Mupirocin, a clinically used natural antibiotic, inhibits isoleucyl-tRNA synthetase (IleRS), an enzyme that links isoleucine to its tRNAIle for protein synthesis. Two IleRSs, mupirocin-sensitive IleRS1 and resistant IleRS2, coexist in bacteria. Specifically, type 1 proteins (IleRS1) are strongly inhibited by mupirocin (Ki in low nanomolar range), while IleRS2, which are homologous to IleRSs from the eukaryote cytosol, exhibit resistance to mupirocin concentrations that are about three orders of magnitude higher. AARSs catalyze the formation of AA-tRNA in two steps within the same active site. The amino acid is first activated by ATP to form an aminoacyl-adenylate (AA-AMP) intermediate, followed by the transfer of the aminoacyl moiety to the tRNA.

To understand how IleRS2, but not IleRS1, accommodates the non-canonical motif, we used X-ray crystallography to determine the structures of a pair of IleRS enzymes from the same organism. Apart from wild-type PmIleRS1 and PmIleRS2, both of which harbor the canonical HXGH motif, we also structurally characterized their corresponding GXHH mutants, all in complex with a non-hydrolyzable analog of the isoleucyl-adenylate reaction intermediate, Ile-AMS. Additionally, the structure of the C-terminal tRNA anticodon binding domain, which differs among the two IleRS types, is resolved for a type 2 protein. However, superimposing the HUP catalytic cores of IleRS1 (residues 50–174 and 523–635) and IleRS2 (residues 40–168 and 513–632) unraveled conformational rearrangements within the signature motifs in the active sites. Relative to IleRS1, the KMSKS loop assumed a more closed conformation in IleRS2, as indicated by a 5.0 Å displacement of the first Lys backbone towards helix α1. While the KMSKS loop is known to be flexible and to change its conformation during the reaction, we also found that the HXGH motif in IleRS2 is displaced towards the KMSKS loop. The latter affects repositioning of the first and the fourth histidine of the HXGH motif by 2.3 and 2.4 Å, respectively, and the Gly α-carbon by 1.7 Å relative to the analogous positions in IleRS1 (insets). The displacement (shift) of the HIGH motif in IleRS2 is of utmost importance for the accommodation of the non-canonical A/GXHH motif and emergence of hyper-resistance.

> MKEVNVRESSQEREQRIQQQWQKGNVFQQSVQNREGYPSFVFYEGPPTANGLPHVGHALGRTIKDVVARYKTMTGHQVIRKAGWDTHGLPVELGVEKQLGISGKHDIEKYGVEAFINKCKESVFVYEKQWRTFTEQLGYWVDMEDPYITLENSYIESVWNVLGTIHDKGLLYKGHRVSPYCPSCQTSLSSHEVAQGYKDVKDLTVTVKFKVKNRDNEYFLGWTTTPWTLPSNVALAVHEEMSYVRAEQGDSVYIVAEALADKVLKGEYSVLSHHKGNELKGMSYEPPFNFVKVEKGHEVVTADYVTDQSGTGVVHLAPAYGEDDYRVVKENGFSFVNVVDEKGQYTSEVPPFQGRFVKDCDVDIVRYLANQDVLYHKEKHEHSYPFCWRCDSPLLYYANESWFIQTTALKEQFLKNNESVKWYPDHIKHGRFGKFLENMVDWNISRKRYWGTPLNVWECEGCQHQVAPKSIKELQKHASHYVDDSIELHKPYVDDVQLTCPVCSGEMKRTPEVIDVWFDSGSMPFAQYHYPFENSELFQKQFPADVIAEGIDQTRGWFYSLMAVSTLFTGKAPYKRVLSLGHVLDENGQKMSKSKGNALDPVDLIHTFGADALRWALLADSAPWNPKKFSERVVQEAKSKVIDTLVNVYGFYVLYAKLDGYDPEQTYELKKTKLDEWILSRLHSTVKRATVHLEDYGFTSAAREIAVFIEELSNWYVRRSRDRFWSEGMDGEKAAAYDTLHEVLVTLSQLLAPFTPFVADDVHENLTGKSVHLADYPACDQTKVNEKLEKEMAAVLQVVELGRSIRNTHSLKVKQPLQSLSLVVTEEDVEWKAYRDVIKDELNVKNFNVEQDDDKLVSYVLKLDFKQAGPKFGKQVNEVNQALKNLSEEKGKEFVEQGKLSVTLASGENLTLETEDVLVEKVPKEGFAVASNGMYTAVLDTALTEELVQEGVAREVIRAVQDYRKKLDLPVNSRINLELSGDEEVQKAVAKFETLLQENLLLHSLSVKETIKNGETVKVGTKQVVLRVLNQS> MSGIALSRLAQERKAWRKDHPFGFVAVPTKNPDGTMNLMNWECAIPGKKGTPWEGGLFKLRMLFKDDYPSSPPKCKFEPPLFHPNVYPSGTVCLSILEEDKDWRPAITIKQILLGIQELLNEPNIQDPAQAEAYTIYCQNRVEY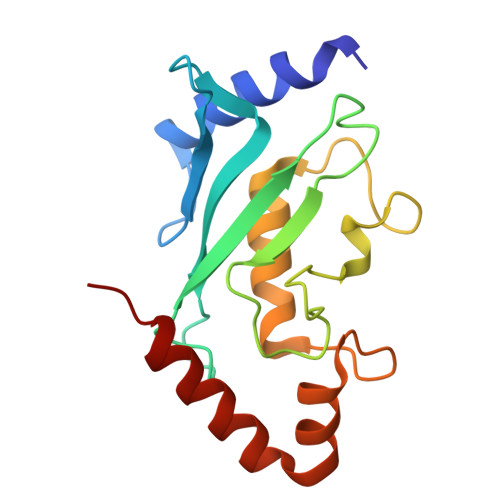EKRVRAQAKKFAPS>[26x]MSAKVKKPELLIFDVNETLLDMGPLENAINESLNSEHAFSLWFRTLLHYSLTETLTGNYVDFGTIGKATLKMTMRKFGKNLSEDRLDAILGNIKKLPAHEDVKEGLKMLKEAQI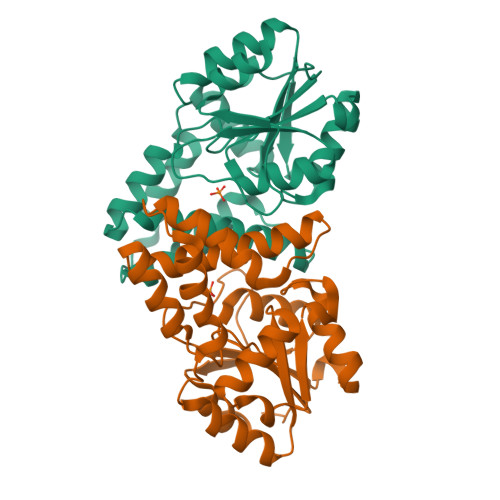KLVALSNSNGKLLNAQLQFAGLADYFDAIFSVEAVGRYKPELASYRAVLETMKVPAENTMMVAANGWDILGAKRAGLRTAFVAREGHAIYPLDGTPELEAKTVLEVARTLLKN>[4x]FQSDKAAEEIDPPQDVTFVNDEAGANSNTTAAKKTESEKSDTAKADQASSTVMRELYLIDKNGYVVAQTLPLPKSESTAKQALEYLVQGGPVSEILPNGFRAVLPADTTVNVDIKKDGTAIADFSNEFK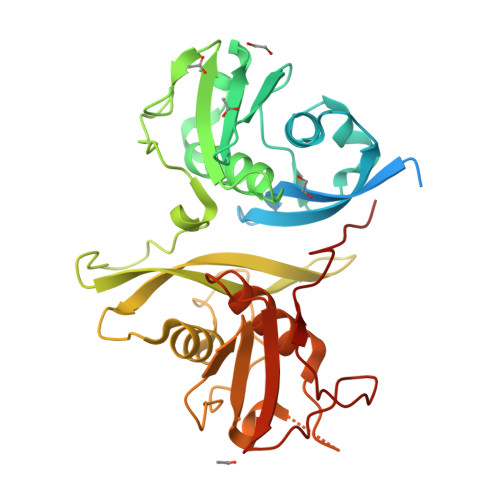NYKKEDEQKIVQSVTWTLTQFSSIDKVKLRINGHELKEMPVGGTPISDDLSRKDGINLETAGVNDLTATHPLTVYYLAENEDSEYYVPVTKRIDNSEKDDITAAINELAKGPSKVSGLLTDFSEDVKLVSKPKIKDGRVTLDFNQSIFGSADEKTKMISSEVLNSIVLTLTEQPDVKSVSVKVNGKSELVNEKGEKLTEPVSRPSQVNTGSF> GGGGGMNGGPGMDGTSEVDLSGAGSPVGAAGWRVDPWIFWAKWGSGPDLGWHPLLCHMLDVAAVTLQMWRRVLPAAWKARISGVLGVGQEDAERWLAFFAGGHDIGKASPAFQLQLRPEQGRELVARRLRDAGLPLFNARAPHGTISANVLETVLADVFGLSGRSARWVAFAVGGHHGFVPSYDEVRRDLDQQAVGWGMWDAAREVLLCRLADALGLPGSSRPTVESTPDAFMLAGLVSVADWIGSNEEYFPYAAQSALQVPQLDAEAYLERAMRQAERAMASLGWVGWRPASGSMRLTELFPYIRQ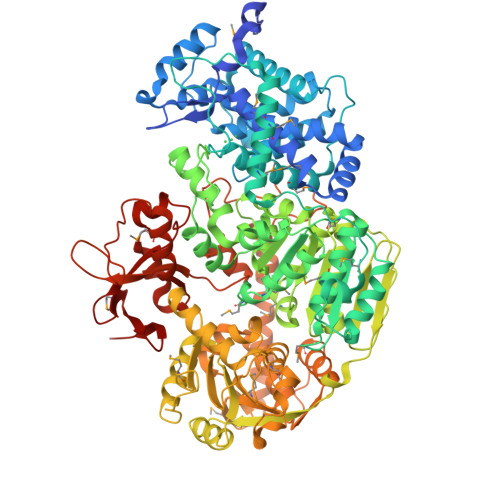PTTVQAAAEELAGEVKSPSITIIEAPMGEGKTEAAMLLADTFSTAHGMSGCYFALPTMATSNQMFGRVTDYLRHRYPEDVVVVNLVHGHSDLSALLQELRQKGEEIFQLQGVYDEALGDEQLGAVVAGQWFTRGKRALLPPYGVGTVDQALLAVLQVKHVFVRLFALSTKTVIVDEVHAYDVYMTTLLHRLLEWLGALSVPVVVLSATLPSARRRELVKAYARGAGWQAERDLPPAGYPRITYAAAEDVRGIHFAPSEASRRKVALRWVSAPEHEALGQLLAEALSQGGCAAIICNTVPRAQALYSALREVFPGLAEDGMPELDLLHARYPYEEREVREARTLGRFSRNGRRPHRAILVATQVIEQSLDLDFDLMVTDLAPVDLVLQRMGRLHRHPVHDPLRPERLRSPELWVVSPQVMGDVPIFDRGSASVYDEHTLLRSWLALRDRDTLQLPEDIEELVEQVYSDGRVPQGASEELRSLWERTFKAQQKVLREDSLQAKYRYIKGPGYNSIWGIVTASVEEDAPELHPALQALTRLAEPSVSAVCLVAGSGGPCLPDGTPVDLDTPPDAAMAERLLRRSVAITDARVLDPLLDVPVPKGWERSSLLRGYRPLVFDASGRAMVGRWIVRIDPELGIVVESP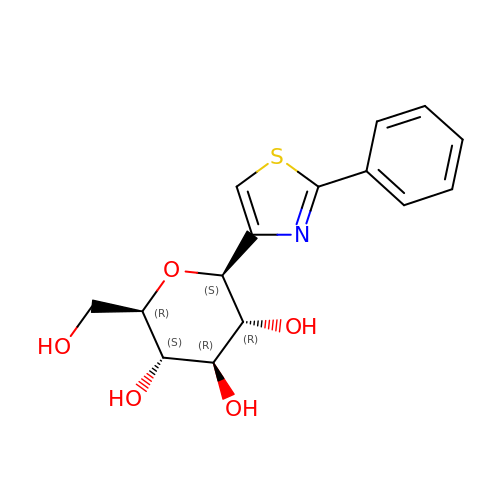(2~{R},3~{S},4~{R},5~{R},6~{S})-2-(hydroxymethyl)-6-(2-phenyl-1,3-thiazol-4-yl)oxane-3,4,5-triol | C15 H17 N O5 S | PFYRBHFULSKLRW-RGDJUOJXSA-N>[3x]SMTGAVCPGSFDPVTLGHLDVFERAAAQFDEVIVAVLINPNKAGMFTVDERIEMIRESTADLPNLRVESGQGLLVDFVRERGLNAIVKGLRTGTDFEYELQMAQMNKHIAGVDTFFVATAPAYSFVSSSLAKEVATYGGDVSALLPASVHQRLLGKLRGQAQ

In this study, we explore M. abscessus phosphopantetheine adenylyl transferase (PPAT), an enzyme involved in the biosynthesis of Coenzyme A, as a target for the development of new antibiotics. Phosphopantetheine adenylyltransferase (PPAT or CoaD) catalyses the penultimate step in the biosynthesis of CoA in prokaryotes. The enzyme catalyses the reversible transfer of an adenylyl group from ATP to 4′-phosphopantetheine (PhP) to yield 3′-dephospho-CoA (dpCoA) and pyrophosphate. Further studies on M. tuberculosis show the essential role played by the coaD gene in mycobacterial growth in vitro, confirming the potential of PPAT as an antibiotic target.

Screening of a fragment library of 960 molecules by differential scanning fluorimetry and hit validation using X-ray crystallography resulted in the identification of 16 fragment hits. These fragment hits occupy four distinct sub-pockets in Mab PPAT, spanning the entire active site groove of the enzyme thus providing several potential starting points for drug discovery. Although the corresponding prazole fragment 1 occupies sub-pocket I on Mab PPAT, the indole fragment 5 preferentially binds sub-pocket III, as do the indole fragments 7 and 12 on Mab PPAT. Fragment interactions at sub-pockets III and IV coincide with the binding mode of Mab PPAT in complex with PhP. Therefore, crucial contacts at this part of the active site, such as those mediated by Leu72-73, Leu36, Pro7, Ser9 and Glu132, were recapitulated by these fragments. Sub-pocket III is seen in an occluded state in apo, and native ligand bound Mab PPAT structures. Whereas fragment binding results in an open conformation allowing further chemical exploration of this cryptic site.>[2x]SGAHMTRNGPGQTTGHPYYLRSFLVVLKTVLENEDDMLLFDEQEKGIVTKFYQLSATGQKLYVRLFQRKLSWIKMTKLEYEEIALDLTPVIEELTNAGFLQTESELQELSEVLELLSAPELKSLAKTFHLANPNGQKQQLVDAFLKLAKQRSVIGAVILKRAKALAGQSVRICKGPR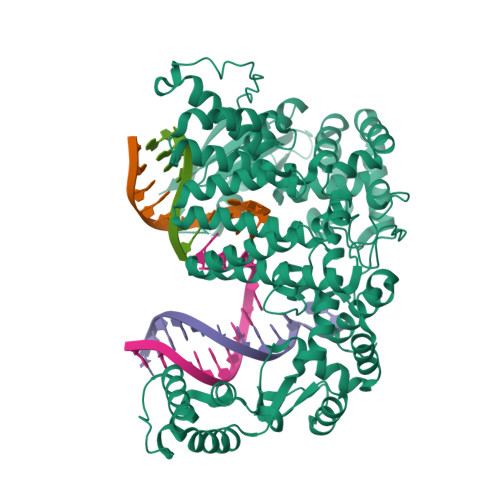AVFSRILLLFSLTDSMEDEDAACGGQGQLSTVLLVNLGRMEFPSYTINRKTHIFQDRDDLIRYAAATHMLSDISSAMANGNWEEAKELAQCAKRDWNRLKNHPSLRCHEDLPLFLRCFTVGWIYTRILSRFVEILQRLHMYEEAVRELESLLSQRIYCPDSRGRWWDRLALNLHQHLKRLEPTIKCITEGLADPEVRTGHRLSLYQRAVRLRESPSCKKFKHLFQQLPEMAVQDVKHVTITGRLCPQRGMCKSVFVMEAGEAADPTTVLCSVEELALAHYRRSGFDQGIHGEGSTFSTLYGLLLWDIIFMDGIPDVFRNACQAFPLDLCTDSFFTSRRPALEARLQLIHDAPEESLRAWVAATWHEQEGRVASLVSWDRFTSLQQAQDLVSCLGGPVLSGVCRHLAADFRHCRGGLPDLVVWNSQSRHFKLVEVKGPNDRLSHKQMIWLAELQKLGAEVEVCHVVAVGAKSQSLS>AMGSRLYDRRSIFDAVAQSNCQELESLLPFLQRSKKRLTDSEFKDPETGKTCLLKAMLNLHNGQNDTIALLLDVARKTDSLKQFVNASYTDSYYKGQTALHIAIERRNMTLVTLLVENGADVQAAANGDFFKKTKGRPGFYFGELPLSLAACTNQLAIVKFLLQNSWQPADISARDSVGNTVLHALVEVADNTVDNTKFVTSMYNEILILGAKLHPTLKLEEITNRKGLTPLALAASSGKIGVLAYILQREIHEPECRHLSRKFTEWAYGPVHSSLYDLSCIDTCEKNSVLEVIAYSSSETPNRHDMLLVEPLNRLLQDKWDRFVKRIFYFNFFVYCLYMIIFTAAAYYRPVEGLPPYKLKNTVGDYFRVTGEILSVSGGVYFFFRGIQYFLQRRPSLKSLFVDSYSEILFFVQSLFMLVSVVLYFSQRKEYVASMVFSLAMGWTNMLYYTRGFQQMGIYAVMIEKMILRDLCRFMFVYLVFLFGFSTAVVTLIEDGKYNSLYSTCLELFKFTIGMGDLEFTENYDFKAVFIILLLAYVILTYILLLNMLIALMGETVNKIAQESKNIWKLQRAITILDTEKSFLKCMRKAFRSGKLLQVGFTPDGKDDYRWCFRVDEVNWTTWNT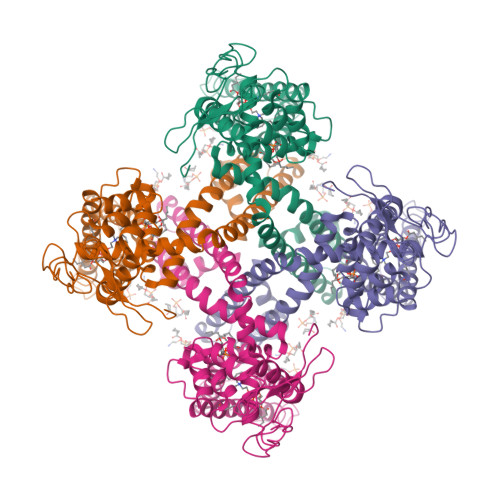NVGIINEDPG[4x]>TRKTYTLTDYLKNTYRLKLYSLRWISDHEYLYKQENNILVFNAEYGNSSVFLENSTFDEFGHSINDYSISPDGQFILLEYNYVKQWRHSYTASYDIYDLNKRQLITEERIPNNTQWVTWSPVGHKLAYVWNNDIYVKIEPNLPSYRITWTGKEDIIYNGITDWVYEEEVFSAYSALWWSPNGTFLAYAQFNDTEVPLIEYSFYSDESLQYPKTVRVPYPKAGAVNPTVKFFVVNTDSLSSVTNATSIQITAPASMLIGDHYLCDVTWATQERISLQWLRRIQNYSVMDICDYDESSGRWNCLVARQHIEMSTTGWVGRFRPSEPHFTLDGNSFYKIISNEEGYRHICYFQIDKKDCTFITKGTWEVIGIEALTSDYLYYISNEYKGMPGGRNLYKIQLSDYTKVTCLSCELNPERCQYYSVSFSKEAKYYQLRCSGPGLPLYTLHSSVNDKGLRVLEDNSALDKMLQNVQMPSKKLDFIILNETKFWYQMILPPHFDKSKKYPLLLDVYAGPCSQKADTVFRLNWATYLASTENIIVASFDGRGSGYQGDKIMHAINRRLGTFEVEDQIEAARQFSKMGFVDNKRIAIWGWSYGGYVTSMVLGSGSGVFKCGIAVAPVSRWEYYDSVYTERYMGLPT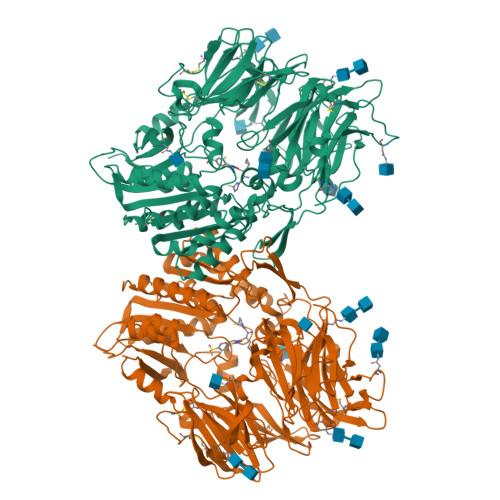PEDNLDHYRNSTVMSRAENFKQVEYLLIHGTADDNVHFQQSAQISKALVDVGVDFQAMWYTDEDHGIASSTAHQHIYTHMSHFIKQCFSLP[2x]> AEIYNKDGNKVDLYGKAVGLHYFSKGNGENSYGGNGDMTYAALGFKGETQINSDLTGYGQWEYNFQGNNSEGADAQTGNKTALAFAGLKYADVGSFDYGRNYGVVYDALGYTNMLPQFGGDTAYSDDFFVGAVGGVATYRNSNFFGLVDGLNFAVQYLGKNERDTARRSNGDGVGGSISYEYEGFGIVGAYGAADRTNLQEAQPLGNGKKAEQWATGLKYDANNIYLAANYGETRNATPITNKFTNTSGFANKTQDVLLVAQYQFDFGLRPSIAYTKSKAKDV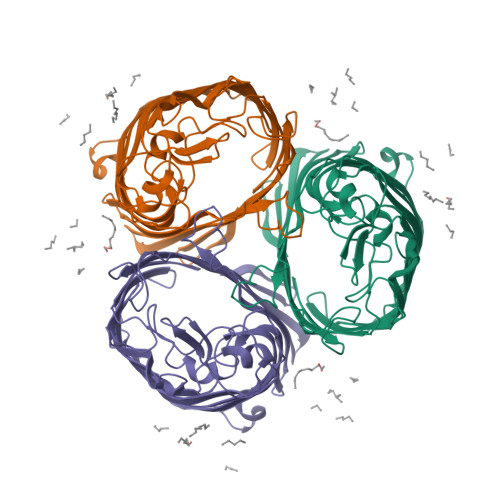EGIGDVDLVNYFEVGATYYFNKNMSTYVDYIINQIDSDNKLGVGSDDTVAVGIVYQF>[2x]GSHMASMSEVERALDVLLQEAEELCIGSSVVELDRIPTALEFCREFYSKNQPVVIRKALNWPAIGKWTPKYLIEALGDRSVDVAITPNGYADGLATQNGQEYFVLPLETKMKLSEVVRRLDDPTGAVHYIQKQNSNLSVDLPELAADLRVSDLDFAQQSFNKPPDAVNFWLGDERAVTSMHKDPYENVYCVISGHKDFVLIPPHQLSCVPRGIYPTGVYKTSDSGQFYIEPLRDEEGSDQFTEWVSVDPLSPDLAKYPEYARAKPLKVRVHAGDILYLPNYWFHHVSQSHKCIAVNFWYDLDYDSRYCYYRMLEQMTSARSG

Jumonji domain-containing 7 (JMJD7) is a JmjC (3S)-lysyl-hydroxylase that catalyses the modification of Developmentally Regulated GTP Binding Proteins 1 and 2 (DRG1 and 2); JMJD7 has also been reported to have histone endopeptidase activity. Here we report biophysical and biochemical studies on JMJD7 from Drosophila melanogaster (dmJMJD7). Like hsJMJD7, dmJMJD7 forms a homodimer with each 316-amino-acid monomer possessing an N-terminal helix-loop-helix-fold domain (aa 1–42) that forms part of the dimerization interface, a core distorted double-stranded β-helix (DSBH, aa 160–294) fold comprising of eight parallel β-strands and an α-helical C-terminal domain (aa 296–310) which is also involved in dimerization. Notably, the crystallographic analyses on dmJMJD7 combined with previously reported crystal structures for hsJMJD720 reveal the unusual dimerization mode of JMJD7, which involves interactions between the N- and C-terminal regions of both dmJMJD7 monomers and is likely conserved in all animals making JMJD7.

We obtained dmJMJD7 crystals of His6-dmJMJD7.Mn complexed with its co-substrate 2OG or co-product succinate; catalytically inert Mn(II) was used instead of the cofactor Fe(II) to block catalysis under aerobic conditions, as was done for hsJMJD720. Comparison of the dmJMJD7 crystal structures reveals a flexible region (aa 123–138) located N-terminal to the DSBH β-strands, which normally forms a loop around the dmJMJD7 active site and is likely involved in induced-fit during substrate binding. Compared to that observed in the dmJMJD7.Mn. OG/succinate/N-oxalylglycine/2,4-PDCA structures, this loop adopts a different conformation and forms a non-DSBH β-strand extending the major DSBH β-sheet in the N-oxalyl-D-alanine and N-oxalyl-D-phenylalanine complexes. Notably, in the 2OG/succinate/N-oxalylglycine complexes, Trp164 is positioned to form a stacking interaction with the methylene groups of 2OG/succinate/N-oxalylglycine; the C4-methylene substitution in N-oxalyl-D-alanine or N-oxalyl-D-phenylalanine compared to N-oxalylglycine prevents this interaction. Tyr123 is one of four dmJMJD7 residues positioned to form H-bonds with the 2OG/succinate/N-oxalylglycine C5-carboxylate.> MTIENTVNSVENLFDTYKLNDTI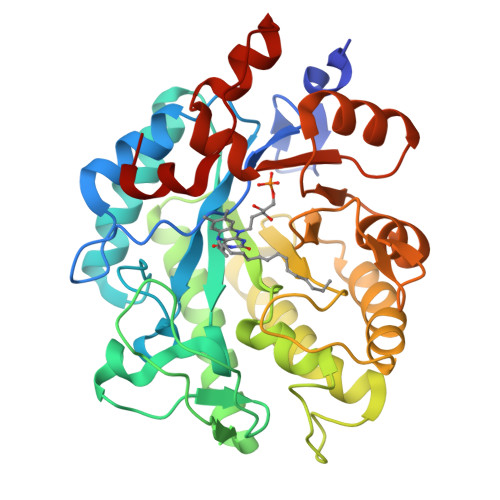TLKNRILMAPLTRCMADANLVPTDDMVAYYARRAEAGLIISEATIIRPDAQGYPNTPGIFTQAQIAGWRKVTDAVHANGGKIFVQLWHTGRVAHPHFFGGGDVLAPSAQKIEGSVPRMRELTYVTPKAVTVEDIQGLVRDYAKAAENVIEAGFDGVEIHGANGYLIDQFLHHDSNRRTDEYGGTPVNMSRFALEVVDAIIARIGHDRTGLRISPGAYFNMASDSRDRVVFDYLLPELEKRDLAFVHIGIFDDSIEFDYLGGTASSYVRAHYGKTLVGVGSYSAETASKAIAEDKFDLIAIGRPFIANPDYVAKVRNSEELVAYSDEMLASLI> RLIEDN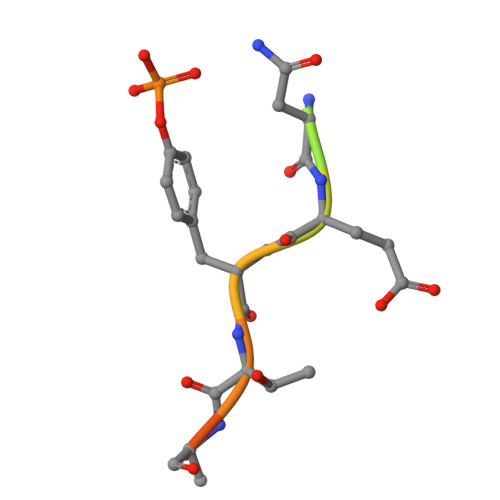EYTARQG N-(7-CARBAMIMIDOYL-NAPHTHALEN-1-YL)-3-HYDROXY-2-METHYL-BENZAMIDE | C19 H17 N3 O2 | 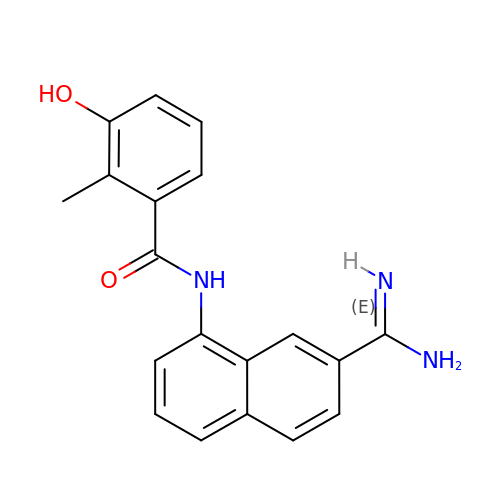NNGZRCYXFBHMRM-UHFFFAOYSA-N> SSQIRQNYSTEVEAAVNRLVNLYLRASYTYLSLGFYFDRDDVALEGVCHFFHELAEEKREGAERLLKMQNQRGGRALFQDLQKPSQDEWGTTL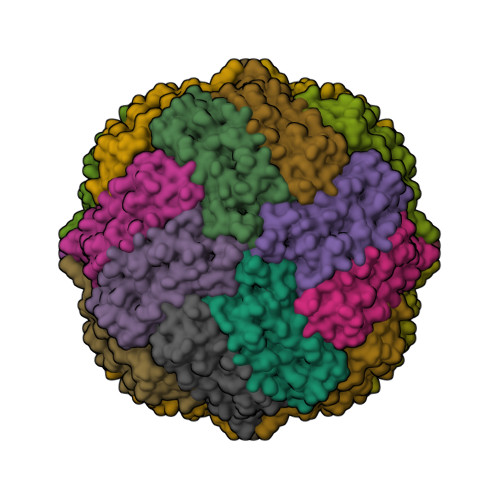DAMKAAIVLEKSLNQALLDLHALGSAQADPHLCDFLESHFLDEEVKLIKKMGDHLTNIQRLVGSQAGLGEYLFERLTLKHD> LYFQGAMALEEIKNGTDISTLDIRKFNLNINNVSVLSKSQSVDQFHLSNPHYEYLSGGAYPGEMENFTLKVDKSKKQDQVFENPLSLKFTNIGTVNGKQVDAYLNFNKVTLHYLNTAQAESEMNSAQKSTVEFFSISELWESNAFEIGNVPYVDANHDYIMNKAFWIDADVTAEIRYADGTETDLKLVMKPTDIDAIDANNLKETFYVKNYQNDVNLRLMNNANVLVQEEASDRTSWIATQITGGSYNENNVSGLALRSNSNSMNFGYSSTETCSAVFGLYIEKIDPRPVLEVDPAEIPAKDGQDVTYKATFKVPVPGKDILAAPSSIEMVQKFDERLDYKELKVESGGVTLQEGRDYTIEKTGQTVTVKMTPEYLKGNSSSDIIITYKTATNKKVEEKGSEKIDNTVTLHVDNLSAPSNQVSTALLYEK;> PTTENLYFQGAMALEEIKNGTDISTLDIRKFNLNINNVSVLSKSQSVDQFHLSNPHYEYLSGGAYPGEMENFTLKVDKSKKQDQVFENPLSLKFTNIGTVNGKQVDAYLNFNKVTLHYLNTAQAESEMNSAQKSTVEFFSISELWESNAFEIGNVPYVDANHDYIMNKAFWIDADVTAEIRYADGTETDLKLVMKPTDIDAIDANNLKETFYVKNYQNDVNLRLMNNANVLVQEEASDRTSWIATQITGGSYNENNVSGLALRSNSNSMNFGYSSTETCSAVFGLYIEKIDPRPVLEVDPAEIPAKDGQDVTYKATFKVPVPGKDILAAPSSIEMVQKFDERLDYKELKVESGGVTLQEGRDYTIEKTGQTVTVKMTPEYLKGNSSSDIIITYKTATNKKVEEKGSEKIDNTVTLHVDNLSAPSNQVSTALLYEK;> IPTTENLYFQGAMALEEIKNGTDISTLDIRKFNLNINNVSVLSKSQSVDQFHLSNPHYEYLSGGAYPGEMENFTLKVDKSKKQDQVFENPLSLKFTNIGTVNGKQVDAYLNFNKVTLHYLNTAQAESEMNSAQKSTVEFFSISELWESNAFEIGNVPYVDANHDYIMNKAFWIDADVTAEIRYADGTETDLKLVMKPTDIDAIDANNLKETFYVKNYQNDVNLRLMNNANVLVQEEASDRTSWIATQITGGSYNENNVSGLALRSNSNSMNFGYSSTETCSAVFGLYIEKIDPRPVLEVDPAEIPAKDGQDVTYKATFKVPVPGKDILAAPSSIEMVQKFDERLDYKELKVESGGVTLQEGRDYTIEKTGQTVTVKMTPEYLKGNSSSDIIITYKTATNKKVEEKGSEKIDNTVTLHVDNLSAPSNQVSTALLYEK;> ALEEIKNGTDISTLDIRKFNLNINNVSVLSKSQSVDQFHLSNPHYEYLSGGAYPGEMENFTLKVDKSKKQDQVFENPLSLKFTNIGTVNGKQVDAYLNFNKVTLHYLNTAQAESEMNSAQKSTVEFFSISELWESNAFEIGNVPYVDANHDYIMNKAFWIDADVTAEIRYADGTETDLKLVMKPTDIDAIDANNLKETFYVKNYQNDVNLRLMNNANVLVQEEASDRTSWIATQITGGSYNENNVSGLALRSNSNSMNFGYSSTETCSAVFGLYIEKIDPRPVLEVDPAEIPAKDGQDVTYKATFKVPVPGKDILAAPSSIEMVQKFDERLDYKELKVESGGVTLQEGRDYTIEKTGQTVTVKMTPEYLKGNSSSDIIITYKTATNKKVEEKGSEKIDNTVTLHVDNLSAPSNQVSTALLYEK

The Sgo0707 protein consists of 1643 amino acids including a leader peptide, an N-terminal region, eight 84-amino acid repeat domains, five 88-amino acid repeat domains and a C-terminal domain containing the LPXTG sorting motif. Based on their related domain organization, our hypothesis was that the N-terminal region of Sgo0707 also represents an adhesive domain. Interestingly, binding to type-1 collagen was significantly reduced in the mutant strain. These data suggest that Sgo0707 plays a role in initial adherence of S. gordonii to type-1 collagen. Interactions between the wild-type strain and collagen-coated surfaces could be competitively inhibited using a recombinant polypeptide encompassing residues 36–458 of Sgo0707, suggesting that binding is mediated via the N-terminal region.

The structure of S. gordonii Sgo0707N was solved to a resolution of 2.4 Å by single anomalous dispersion using one crystal of SeMet substituted protein belonging to the I222 space group with four molecules in the asymmetric unit. The initial model was subsequently refined against native data to 2.1 Å resolution. The structure can be divided into two domains, N1 and N2, which both adopt β-sandwich folds with antiparallel β-sheets. The N1-domain is the largest domain (residues 36–311) harbouring a putative binding cleft which strengthens the original hypothesis of the N-terminal, non-repetitive domain, functioning as an adhesin. The pocket exhibits a predominantly negative surface potential formed by Glu81, Glu169, Glu174, Glu232, Asp221, Asp223, Glu277, Glu300 together with the polar residues Thr220, Asn278 Ser274, Ser303 and Cys302. In all four chains positive electron density is found in the cleft but this is more pronounced in chains A and D. Although the protein was crystallized without the addition of metal ions positive electron density, indicating a partly occupied metal ion was observed in association with Asp221 (OD1), Asp223 (OD2) and Thr271 (O) of the A-chain. Interestingly, the 1643 amino acid long protein contains only one cysteine, Cys302, and that single residue is located in the floor of the putative binding cleft in the N1-domain. To our surprise we found that the N1-domain, despite very low sequence similarity, exhibits a striking structural similarity to the variable domains of the AgI/II adhesins, also expressed by oral streptococci. Whereas the Sgo0707 cleft is predominantly negatively charged the AgI/II clefts are less charged and have a tightly bound metal ion. No isopeptide bonds are however observed in the Sgo0707 N2-domain and the residues in the equivalent lysine-asparagine positions are Leu319 and Asn434.>[2x]KELLDSDGDILRNGGTYYILPALRGKGGGLELAKTGDETCPLNVVQARSETKRGRPAIIWTPPRIAILTPAFYLNIEFQTRDLPACLEEYSRLPWKVEGESQEVKIAPKEEEQHLFGSFKIKPYRDDYKLVYCEGNSDDDSCKDLGISIDDENNRLLVVKDGDPLAVRFVKAHRRG

The plant protease inhibitor EcTI from Enterobobium contortisiliquum is a classical trypsin inhibitor belonging to the Kunitz family. A Kunitz-type inhibitor that was first isolated from Enterolobium contortisiliquum was named EcTI. It was shown that EcTI inhibits trypsin, chymotrypsin, plasma kallikrein, plasmin, human neutrophil elastase, and Factor XIIa in the stoichiometric ratio 1∶1, but not thrombin, bovine pancreatic elastase, or Factor Xa. The fold of EcTI is a β-trefoil, typical for the STI-related family of Kunitz inhibitors. As found in most known Kunitz-type inhibitors, EcTI has a single reactive site located on loop L5, between β-strands 4 and 5.

In this work, we investigated the structural basis of the activity of EcTI by determining its crystal structure in the unbound and trypsin-bound form. The structure of free EcTI was refined to a higher resolution of 1.75 Å. The final model contains two inhibitor molecules, two imidazole molecules, two glycerol molecules, and 244 water molecules. Molecule A consists of residues 1–134 and 141–174, whereas molecule B contains residues 1–134 and 141–173. A loop region containing residues 23–26 of monomer B is in weak electron density, but is still included in the final model, whereas the density for the loop containing residues 111–113, not traced in the complex, is very clear. A molecule of EcTI contains two disulfide bonds, one intra-chain and one connecting two chains. However, since the crystal structures of EcTI were obtained under mildly reducing buffer conditions, the disulfide bond Cys40-Cys86 was broken in molecule A of the free EcTI, as well as in the inhibitor molecule in the EcTI-trypsin complex. This observation indicates that the disulfide bond Cys133-Cys142 plays a more important role in stabilizing the β-trefoil fold, whereas the disulfide bond Cys40-Cys86 may not be as necessary for its stability. The equivalent residue in EcTI is also Asn13, which similarly forms a network consisting of several hydrogen bonds. Taking monomer B of free EcTI as a reference, only the Cα atoms of the P1, P2, and P1′ residues exhibit minor shifts, whereas the remaining residues of the reactive loop are in almost exactly the same conformation.> GNLYTWGQYASGTGFETASAVPRKVDYFSGNVSKVAMGPYHTAVITNDGSLYTFGWGQNGALGNGAKEFQLSPSPVSFFNDKKLKVKDVVVGESYTIAVTENGEVYSWGYGGEPSSKINLDFFRNAILPQRCGALGSGDNKNRLTPQQIANLKADGYKNISGGDNFATLVNQSGEVINWGTGLFGSLGNGSDYPLFTPEVNAYFKHLKE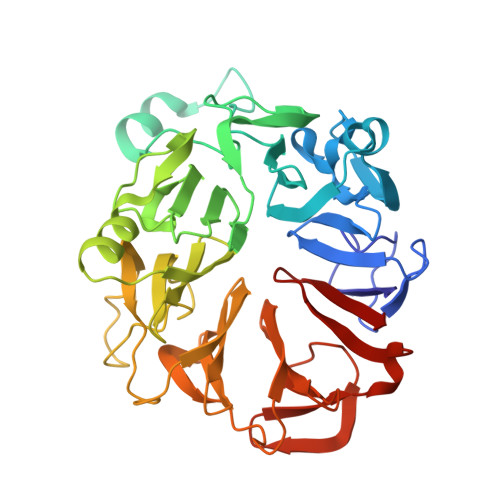HEGLTVQSIKSAGHFSAALLSNGKLYTFGVNTQGQLGIRENLGHNTDQNARLPTPVVDRHFVGQKVVDFEVGENTLVFLTDKNEVFFSGLELAYQPIRWEIPTDKKIVKLAASKDTFAAVTETGKIYQFNEFVGVSTNEVGNDYNVADSKAFEGKVVDLGGSYGIRFAIVN[2-methyl-5-(trifluoromethyl)pyrazol-3-yl]boronic acid | C5 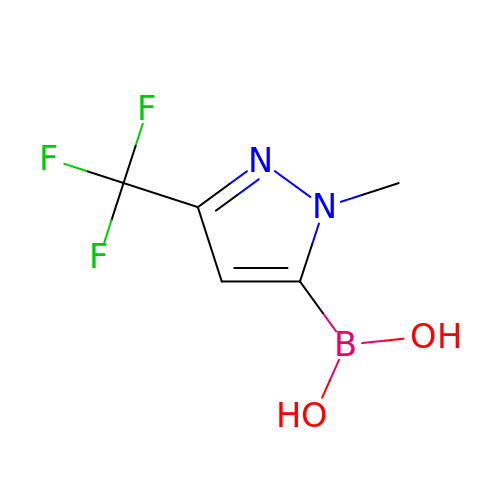H6 B F3 N2 O2 | XPUNXPPXMANQGF-UHFFFAOYSA-N> MAHSKHGLKEEMTMKYHMEGCVNGHKFVITGEGIGYPFKGKQTINLCVIEGGPLPFSEDILSAGFMYGDRIFTEYPQDIVDYFKNSCPAGYTWGRSFLFEDGAVCICNVDIT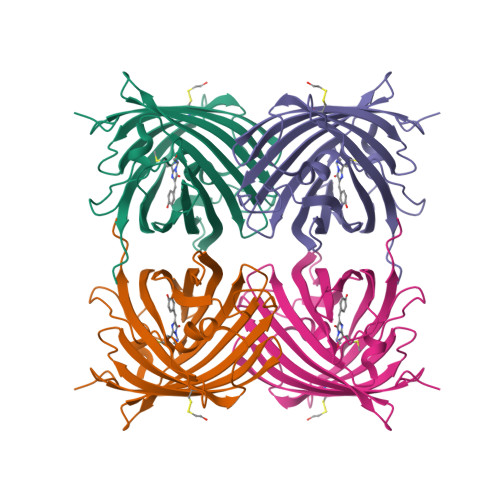VSVKENCIYHKSIFNGMNFPADGPVMKKMTTNWEASCEKIMPVPKQGILKGDVSMYLLLKDGGRYRCQFDTVYKAKSVPSKMPEWHFIQHKLLREDRSDAKNQKWQLTEHAIAFPSALA>MRIPLVGKDSIESKDIGFTLIHEHLRAFSEAVRQQWPHLYNEDEEFRNAVNEVKRAMQFGVKTIVDPTVMGLGRDTRFMEKVVKATGINLVAGTGIWIFIDLPFYFLNRSIDEIADLFIHDIKEGIQGTPNKAGFVKIAADEPGITKDVEKVIRAAAIANKETKVPIITHSNAHNNTGLEQQRILTEEGVDPGKILIGHLGDTDNIDYIKKIADKGSFIGLDRYGVDLFLPVDKRNETTLRLIKDGYSDKIMISHDYCCTID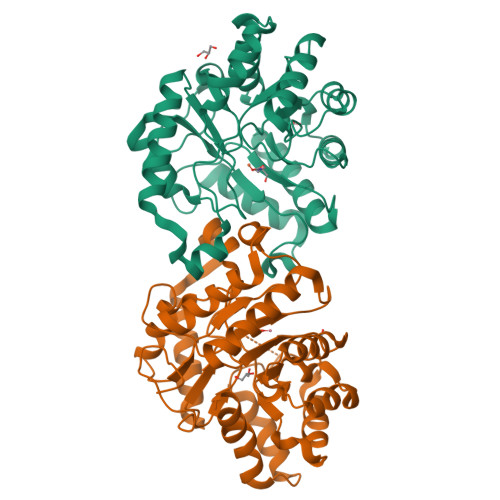WGTAKPEYKPKLAPRWSITLIFEDTIPFLKRNGVNEEVIATIFKENPKKFFS[4x]> GMSLANQIDQFLGTIMQFAENKHEILLGKCESDVKLTSTQAHILMLLAEQISTNAKIAEKLKISPAAVTKALKKLQEQELIKSSRATNDE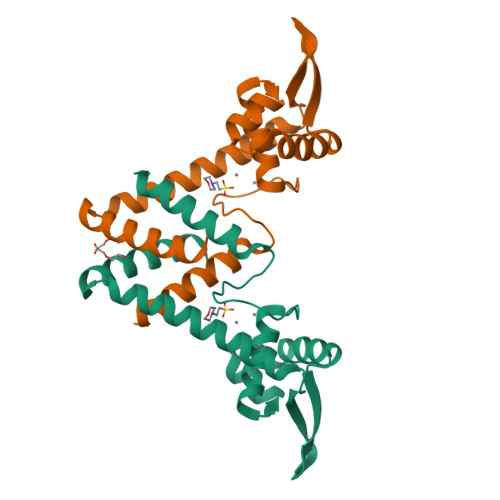RVVLWSLTEKAVPVAKEHATHHEKTLSTYQELGNKFTDEEQEVISKFLSALTEEFQ> MINISAFGSICQFTASRTFPNGFTVTEFADDADPIDSPPFTAADTGVGLNGDMVVWNRANILEVVVNVIPNTE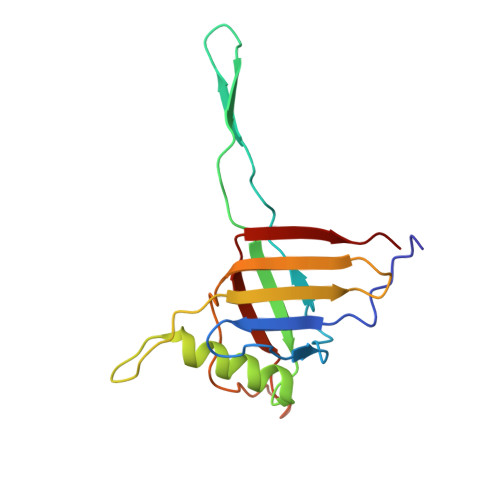GERNLAVLLDANRTGKDKSGARDVVGLVVAMPDGSKITCTNGTPIDGVLINAVASVGRLKTKPYRFRFEKVIKAGTS> SGTGLGEVDVDTYLSNLQTKTT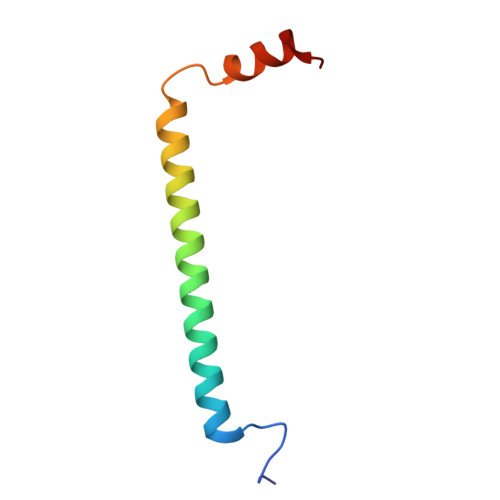LSMIADGLERSARDFDAFLEENVTLEWEAQRKRIYQHFGIK>ASAKELACQEITVPLCKGIGYQYTYMPNQFNHDTQDEAGLEVHQFWPLVEIQCSPDLKFFLCSMYTPICLEDYKKPLPPCRSVCERAKAGCAPLMRQYGFAWPDRMRCDRLPEQGNPDTLCMDHHHHHH[4x];>GGVSFSEVMGKQKDEQAREQLKEGMIKIEEQG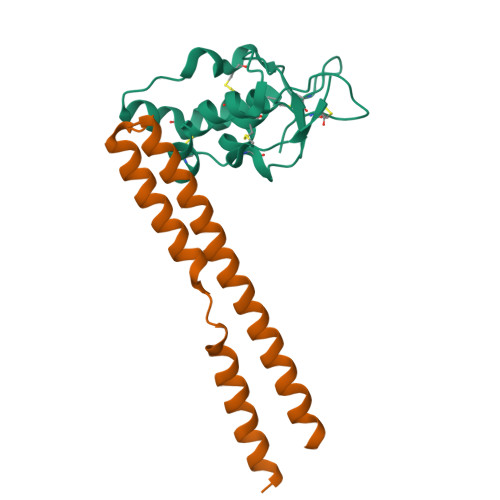KKLSETRTQEELQKYVAAVATFALQAGFLGPNLEERRGFNRRGKEEIGKISGEVYLKLLDLKKAVRAKEKKGLDILNMVGEIKGTLERVYA[4x]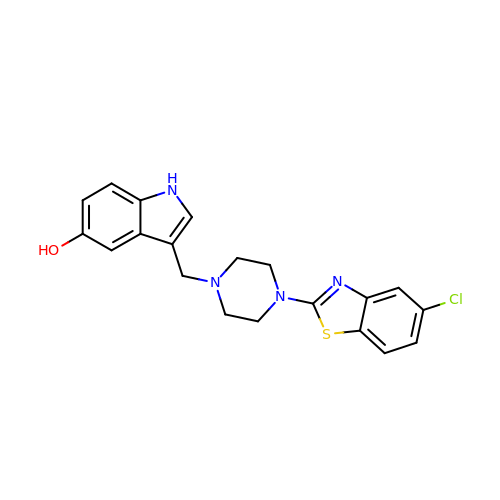3-[[4-(5-chloranyl-1,3-benzothiazol-2-yl)piperazin-1-yl]methyl]-1~{H}-indol-5-ol | C20 H19 Cl N4 O S | HPPQAIGIZOCWPQ-UHFFFAOYSA-N> MATVLTKGEIVLFALRKFAIASNASLTDVEPQSIEDGVNDLEDMMSEWM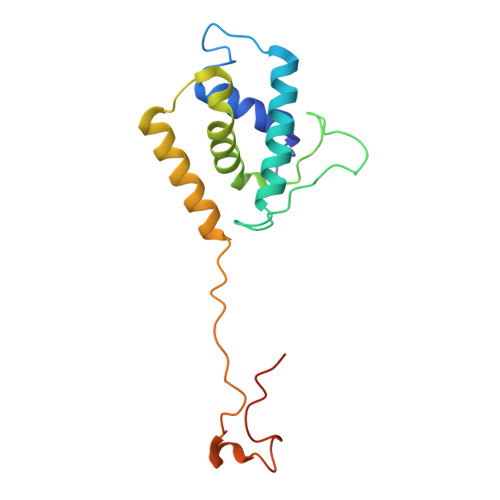INPGDIGYAFATGDEQPLPDDESGLPRKYKHAVGYQLLLRMLSDYSLEPTPQVLSNAQRSYDALMTDTLVVPSMRRRGDFPVGQGNKYDVFTSDRYYPGDLPLIDGDIPNA>[4x]MYEWKLNEIVDSGVCARCGTCTIVCPNGILTFDERPKLIDECLRKGHGMCFEVCPRVSSAKYQIKIREKFYEKYYYAKSDIEGQDGGVVTAFLKYLLENGKIDGAIVVGDECWKPVSLVVQNAEDLLKTAKSKYAISTLDALRKAGEMGLEKVAVVGLPCQINGLRKLQYFPYHAKHDLELGRNGKPVKLPKIEYLIGLFCTEKFRYDNMKEVLSKHGIDIEKVEKFDIKKGKLLVYVNGEKKEFDLKEFEICSGCKMCRDFDAEMADVSVGCVGSPDGYSTIIIRTEKGEEIKNAVELKEGVNLEEIEKLRQLKLKRFKKEVERRRENNEYVSFYWTADYGGIGKRADGTYFIRVRAKPGGWYKPEEIKEILDIAEEYNAKIKVTDRAGYELHGISGFDVEDIVLRLREKGLLTGSEGPLVRATLACPGGGNCSSGLVDTTELARIIEDNFKERPAPYKFKIAISGCPNGCVRPQVHDIGIAGVKYPKVNEEKCNGCGRCAEVCKVEAIDIRGETSYTNYNVCVGCGKCIKNCPNEAREVKEEGYLVYVGGKTGREVVEGVKMKLMSVDEIINFIDKVLVVYGKYAEKPQRERLAAVMKRVGYGKFLEEVKELMKKEIC

Here, we present snapshots of this coupled system, named coenzyme F420-dependent sulfite reductase (Group I Fsr), obtained from two marine methanogens. Fsr organizes as a homotetramer, harboring an intertwined six-[4Fe–4S] cluster relay characterized by spectroscopy. The wire, spanning 5.4 nm, electronically connects the flavin to the siroheme center. Despite a structural architecture similar to dissimilatory sulfite reductases, Fsr shows a siroheme coordination and a reaction mechanism identical to assimilatory sulfite reductases.

A single-wavelength anomalous dispersion experiment was performed to solve the MjFsr crystal structure. The crystal structures of both Fsr superpose well and were refined to 2.30 Å for MjFsr and 1.55 Å for MtFsr. Since MjFsr has pseudo-merohedral twinning and a lower resolution compared to MtFsr, the latter was used for the in-depth structural and biochemical analysis. The binding of the siroheme in MjFsr and MtFsr is highly conserved. On the basis of the observed electron density, we tentatively modeled a SO32− bound to the siroheme iron (2.3 Å) in MjFsr. In MjFsr, four positively charged residues (Arg 355, Arg 423, Lys 460 and Lys 462), which are perfectly conserved across sulfite reductases, bind the SO32− and two water molecules. But both Fsr structures revealed an additional cluster ([4Fe‒4S] cluster 1), which has a noncanonical binding sequence (PCX40CX54CX2C).> GISGRHSITVTTVASAGNIGEDGILSCTFEPDIKLSDIVIQW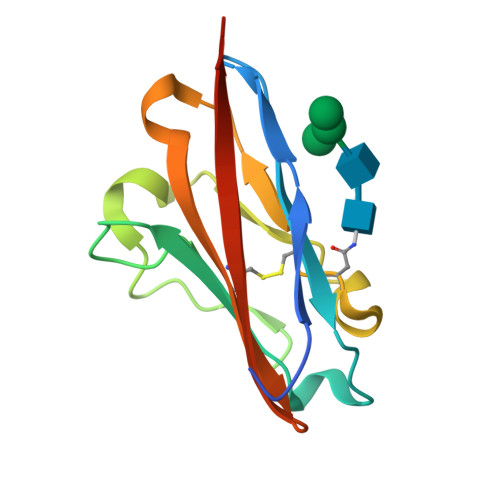LKEGVLGLVHEFKEGKDELSEQDEMFRGRTAVFADQVIVGNASLRLKNVQLTDAGTYKCYIITSKGKGNANLEYKTGHHHHHH> MPRPAPRFAMGHMLPHRSNVGSQFLHTQRHGSRSTWYKKHYFSLRPFAIQRHHGTTPRILLDRSLWKSLWITKLQLPDINRWERVVNSRRVTEDRYAFVEEEGVMHKVNWGLYCER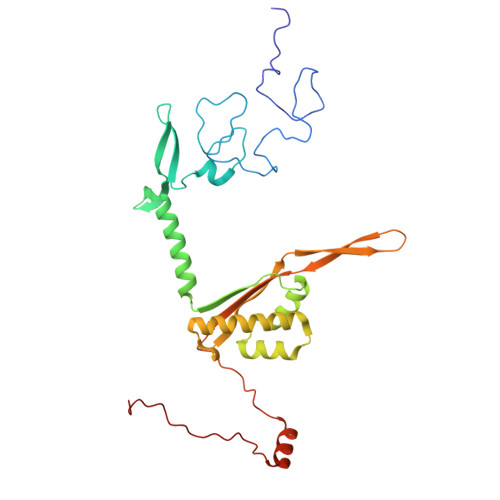LETELTVTQERLPQHTLLMKAVPSSWKKLDIDISVIRGLSLREAMAQCKLSLRKGHQIVFRALEMAQQGAEAKGLDKEHLRVAHISCYPGPTDKQIDIRSKGYYAWKTKKSSHLVLTLAEDPEMVLPDRTCLPYSSLMSMKRAGLSAQPTVIDVPAITADGI> GAMDPRTITMHKDSTGHVGFIFKNGKITSIVKDSSAARNGLLTEHNICEINGQNVIGLKDSQIADIL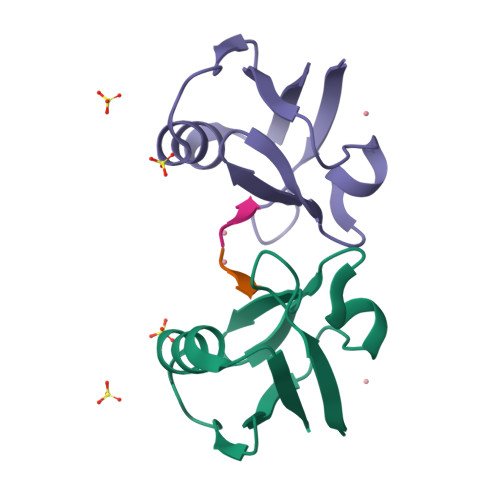STSGTVVTITIM;> ETLEDSVF>MIWTGLLVGFLFGIVLQRGRIAFNSAFRDVLLFKDNYLFKLAVFTLALEMILFVLLSQVGLMQMNPKPLNLVGNIIGGFVFGLGMVLAGGCASGVTYRVGEGLTTAWFAALFYGLGAYATKSGAFSWWLSWVGQFKSPLSVEESAYYVKGAGPTISSVLGLNPWIPALVIAALFILWAFGTKTTSRETKFNWKIASVCLALVAGLGFITSTLSGRKYGLGITGGWINLFQGFLTNSPLNWEGLEIVGIILGAGVAAAVAGEFKLRMPKNPVTYLQVGIGGLLMGIGAVTAGGCNIGHFLTGVPQLALSSWLASIFFILGNWTMAWILFRRAATPTPVAEAAPSSAEDRVLPFQVATGAVALQTAPRVKKAMANYQVSKEIDVRGEVCPIPDVEAKRAVQSANDGEIILVRIDYPLSKERIPETVKKLGSEVLEIEEAAPGEWNIYIKVKKGSSGENLYFQ[2x]

Recently, a selective thiosulfate uptake pathway involving a membrane protein YeeE (TsuA) in Escherichia coli was characterized. Here, we assessed selective thiosulfate transport via Spirochaeta thermophila YeeE in vitro and characterized E. coli YeeD (TsuB) as an adjacent and essential protein for YeeE-mediated thiosulfate uptake in vivo. YeeD is a cytoplasmic protein that belongs to the TusA (tRNA 2-thiouridine synthesizing protein A) protein family. Finally, the crystal structures of S. thermophila YeeE-YeeD fusion proteins at 3.34-Å and 2.60-Å resolutions revealed their interactions.

We succeeded in crystallizing a fusion protein of StYeeE and StYeeD, designed based on the amino acid sequence of Corynebacterium pollutisoli YeeED, which is expressed as a single protein. First, because a comparison of StYeeE/D and several YeeEDs’ amino acid sequences revealed that C. pollutisoli YeeED possesses the shortest linker, of 40 amino acids, between its YeeE and YeeD regions, we prepared the fusion protein by introducing the 40 residues between the C-terminus of StYeeE and the N-terminus of StYeeD. Second, after attempting but failing to crystallize the fusion protein, StYeeE-StYeeD, we tried crystallization using alanine mutants of the conserved cysteines in StYeeE-StYeeD and succeeded in crystallizing StYeeE(C22A)-StYeeD. However, the resolution was insufficient to reveal the details of the interactions between YeeE and YeeD. The asymmetric unit contains 2 molecules of StYeeED, Mol A and Mol B. In the crystal packing, StYeeD in Mol A is involved in interacting with an adjacent YeeD region, but YeeD in Mol B is not. Each crystal lattice in the datasets was the same, except for having slightly different unit cell dimensions. C22 of StYeeE is located at the interface, implying that C22A affects the interaction. From our X-ray crystal structure, YeeE and YeeD appear to work as a 1:1 complex.>[8x]ETQSFNFDHFEENSKELNLQRQASIKSNGVLELTKLTKNGVPVWKSTGRALYAEPIKIWDSTTGNVASFETRFSFNITQPYAYPE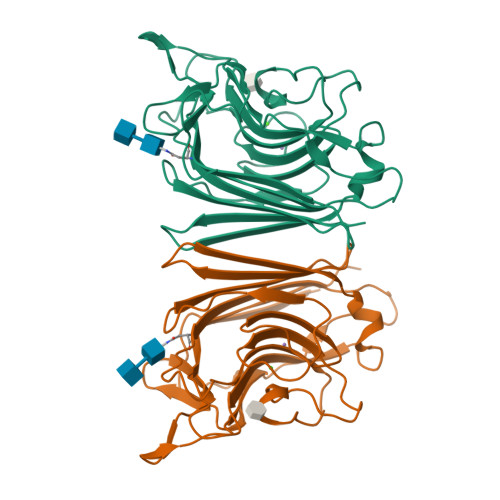PADGLTFFMVPPNSPQGEDGGNLGVFKPPEGDNAFAVEFDTFQNTWDPQVPHIGIDVNSIVSSKTLHFQLENGGVANVVIKYDSPTKILNVVLAFHSVGTVYTLSNIVDLKQEFPNSEWVNVGLSATTGYQKNAVETHEIISWSFTSSLQETN> GDNYADLSDTELTTLLRRYNIPHGPVV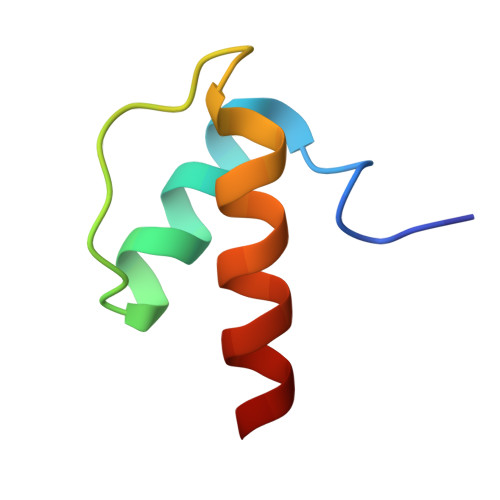GSTRRLYEKKIFEYETQR>MPAAPLDVKCLEANKDYIIISWKQPAVDGGSPILGYFIDKCEVGTDSWSQCNDTPVKFARFPVTGLIEGRSYIFRVRAVNKMGIGFPSRVSEPVAALDPAEKARLKSRPSAPWTGQIIVTEEEPSEGIVPGPPTDLSVTEATRSYVVLSWKPPGQRGHEGIMYFVEKCEAGTENWQRVNTELPVKSPRFALFDLAEGKSYCFRVRCSNSAGVGEPSEATEVTVVGDKLDIP[2x];>GPLGSGILMAPKTFWVNEGKHAKFRCYVMGKPEPEIEWHWEGRPLLPDRRRLMYRDRDGGFVLKVLYCQAKDRGLYVCAARNSAGQTLSAVQLHVKEP[2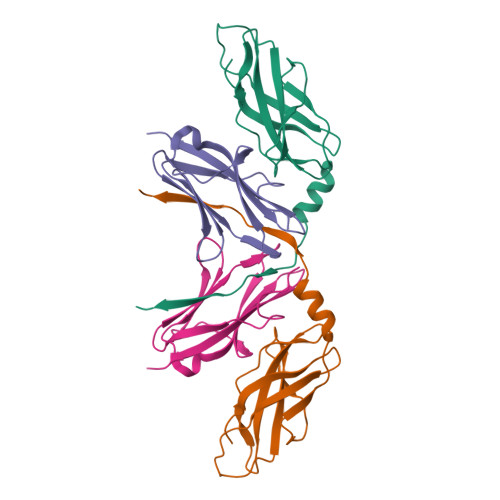x]>[15x]MAIIAGKAGYGLIIALFSLSLSGCGLTQRVADGTVSATKSLFYRQIKTLHLDIRAREAINTSAAGIPLSVVVRIYQLKDNRSFDSADYQALFTGDNEILAGDIIAQKDVWLQPGGSVAVDMPLDDAAKFTGVAAMFLEPDQKKNTWRVVLGRDELEPDTPRLIEVSGNTLTLLPVKDK;>MNKLACLSGRFGRPGIVFIGVAALWWLITRYGAYLGAETRRDQILLLILLSLGVLFVCYLPVMKKY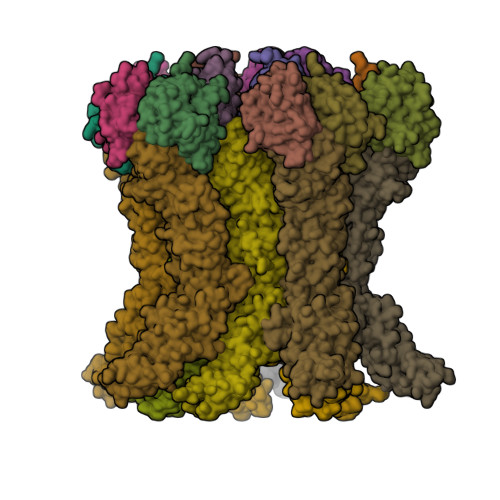VQELTYRRRARKEQRLPDDEERLAQTPPRYVTVQDIRHTLRRQYGRFWGRKIRILLITGTASEVELLTPGLTEQFWQEEQGTLLLWGGDPSQPENADWLAALRRLRYRPADGIVWVTSGLSETLSAPLTEDALDRVSRAVSSCCERLGWRLPLYVWSLQESPDERGRITQPVGCLLPAECSSDKLKAQLQAMLPGLVAQGIQQICCAPRYYFLLSLAERFRRNIDAVVEPLSVLLRPYRQLLLAGIVFSPATVGGERSVRHRWRMDNRWEALPETVQQLPVRLQPSRTGHNWRRSLAVMAAILMMAQGTGMVVSFLANRSLVAEVQEQIRPAQNQQLSPAERLQALLNLQKSLARLQYREEHGAPWYLRAGMNQNADLLAVVMPLYAQNAHLLLRDAAAAHLEQQLRTFIRLPPDSPQRGKMAKAAYDQLRLYLMLAQPQHMEPAWFSRTLMREWPQRDGVSAVFWQANGPTLLAYYASGIITHPQWKLTADEELVSQSRTLLLRHLGTQNSDAMLYQKMLARVAHQFADMRLTDMTGDTDVSRLFFTDEVVPGMFTRQAWEEAVLPSIDTVINERREEMDWVLTDGRQKAPSPVSPEALRQRLTTRYFADFGNAWLNFLNSLHLRKAQTLSDVTEQLTLMADVRQSPLVALMNTLAVQGCTGQPREAVTDSLVKSARNLLSQEKQPVAVPESRLHGPLATTFGPVLALMDNQNNSADMLNLQTYLTRVTQVRLRLQQIAGSSDPQAMMQLLAQTVLQGKSVDLTDTRDYGSLTAAGLGQEWYGFGQTVFVRPMEQAWQQVLTPAAESLNARWRTAVVDGWNNAFSGRYPFKNVSSDASLPLLAKYLNTDTGRIARFLQNNLSGVLHREGSRWVPDTINTRGLTFNPAFLKAINTLSEIADVAFTTGNAGLHFELRPGTAAGVMQTTLITDNQKLIYVNQMPVWKRFTWPADTEAPGASLSWVSTQAGTRQYADLPGSWGLIRLLEMARRKAAPGVASGWSLSWQAQDGRMLNYTLRTEAGEGPLVLLKLRNFVLPETVFELSGTSAFTGNDEDAGDTVEETD[10x]> GHMKKRVGIEALAVAVPSRYVDIEDLAR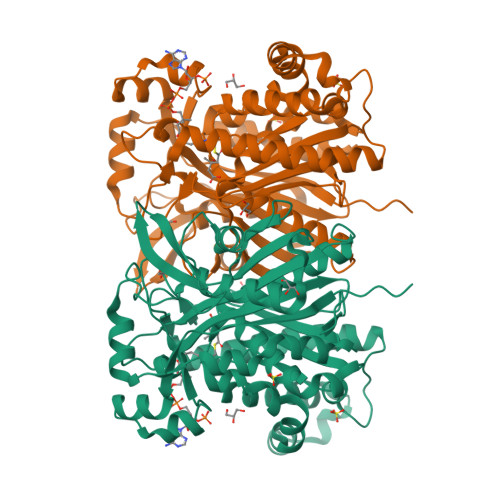ARGVDPAKYTAGLGAREMAVTDPGEDTVALAATAAARLIRQQDVDPSRIGMLVVGTETGIDHSKPVASHVQGLLKLPRTMRTYDTQHACYGGTAGLMAAVEWIASGAGAGKVAVVVCSDIARYGLNTAGEPTQGGGAVALLVSEQPDLLAMDVGLNGVCSMDVYDFWRPVGRREALVDGHYSITCYLEALSGAYRGWREKALAAGLVRWSDALPGEQLARIAYHVPFCKMARKAHTQLRLCDLEDAADAAASTPESREAQAKSAASYDAQVATSLGLNSRIGNVYTASLYLALAGLLQHEAGALAGQRIGLLSYGSGCAAEFYSGTVGEKAAERMAKADLEAVLARRERVSIEEYERLMKLPADAPEAVAPSPGAFRLTEIRDHRRQYAEGN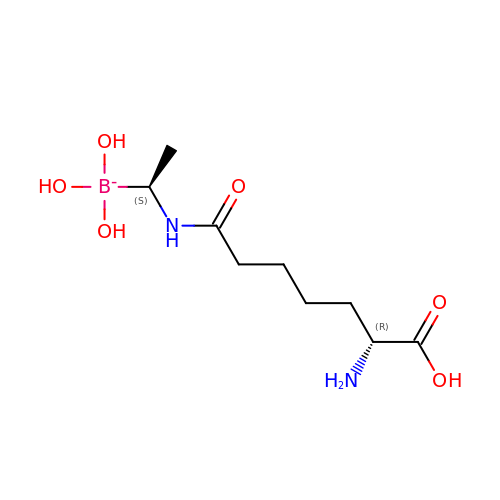(D-ALPHA-AMINOPIMELYLAMINO)-D-1-ETHYLBORONIC ACID | C9 H20 B N2 O6 | ZSMKWHGOAVMEJJ-RNFRBKRXSA-N> MSAP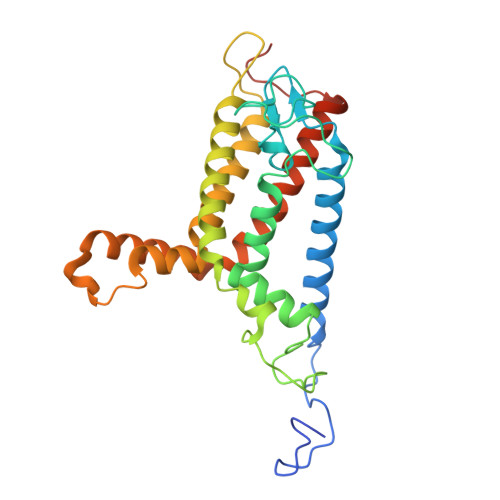TADRRATGVFSPRRAQIPERTLRTDRWWQAPLLTNLGLAAFVIYATIRAFWGSAYWVADYHYLTPFYSPCVSTACAPGSSHFGQWVGDLPWFIPMAFISLPFLLAFRLTCYYYRKAYYRSVWQSPTACAVAEPHAKYTGETRFPLILQNIHRYFFYAAVLISLVNTYDAITAFHSPSGFGFGLGNVILTGNVILLWVYTLSCHSCRHVTGGRLKHFSKHPVRYWIWTQVSKLNTRHMLFAWITLGTLVLTDFYIMLVASGTISDLRFIGHHHHHHHHHH The Neisseriaceae family of Gram-negative bacteria express a bipartite receptor, HpuAB, to efficiently use haem extracted from Hb:Hp complexes as an iron source. HpuA is expressed outside the cell, anchored to the outer membrane by its acylated amino terminus. Although a direct interaction between HpuA on meningococci and Hb was not detected using flow cytometry, the lipoprotein is required for the high-affinity interaction between HpuB and Hb, for meningococcal survival on Hb as a sole iron source and for efficient dissociation of Hb2023. To investigate the structure and function of HpuA we crystallized the carboxy-terminal portion of the protein from N. gonorrhoeae (NgHpuA-C) and a full-length homologue from K. denitrificans (KdHpuA).

We solved the KdHpuA structure by single wavelength anomalous dispersion (SAD) following soaking crystals in cobalt ions. Residues from 15 to 197 and 204 to 322 are visible in the electron density. The structure reveals a single domain composed of a small compact C-terminal β-barrel (residues 157–322) and a more open N-terminal β-sandwich (residues 1–156). Prominent features of the structure include two long extensions from the core of the protein, one formed from two longer strands of the N-terminal β-sandwich (β3 and β4) (loop-1) and the second from a loop at one end of the C-terminal β-barrel, between strands β20 and β23 (loop-5). Both loops present hydrophobic side chains at their distal end including those of Tyr-60, Phe-271 and Tyr-272. A third long loop dividing the second strand of the β-barrel (into β13 and β16) is partially disordered in the structure but also contains the hydrophobic residue Tyr-201 (loop-4). Two shorter loops on the same side of the protein comprise residues 92–100 (loop-2) and 122–127 (loop-3). The B-factors of Gln-123 to Thr-126 of KdHpuA in the unliganded structure are higher than for any other amino acid; further suggesting this is a flexible part of the molecule. Strikingly, although the Cys–Cys motif of TbpB C-lobe has always been observed to form a disulphide bond, in our HpuA structures this motif is in reduced form despite a lack of reducing agent in the protein storage or crystallization buffers. In the KdHpuA apo structure, the region is close to a crystal contact, is poorly defined and probably exists in different conformations, the predominant of which does not include a disulphide; however, in the HpuA:Hb structure, the region is very well defined and neither chain A nor chain B contains a disulphide.

> GPGGTAINEPLTAAPIPVLRAVDTTSPNIVADTSTDREQRTFATQGGSVKPFTITKPSPYIPGLMLTNQEILYQAPDGKYYDFGTYNTLIMPSSSTSARVLPNSHPMQPLDSGGKMIACCTNQTSTGMNALRLKSMQFGAWMSPSKTVSLFAGGTPAPTDTLQGVDTAGRPTGKATYEVIGLRVKNDRAVTSSYETRYSPYNTGQVVTGSFLTVNFNTGKLGGTIVGNSEFGDSIEMRDVNVNGNQFSGTASSGGHTGQVSGGLFAKEERFYSGTLEHPSGGEIGGTVNFGSNSPLNASFGGTRREYNAADTSTDTSHLVSPX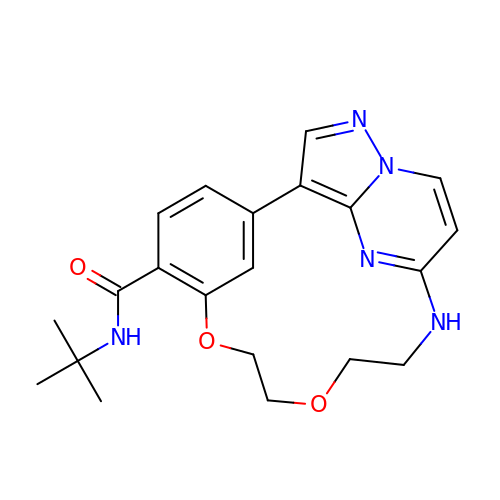~{N}-~{tert}-butyl-7,10-dioxa-13,17,18,21-tetrazatetracyclo[12.5.2.1^{2,6}.0^{17,20}]docosa-1(20),2(22),3,5,14(21),15,18-heptaene-5-carboxamide | C21 H25 N5 O3 | YCFFONJEHNSECY-UHFFFAOYSA-N> MVAESNSAVAPTANVATSPAHEHFVRVNGGHFELQGKPYVITGVNMWYAAYLGAPNEVGDRDRLAKELDNLKAIGVNNLRVLAVSEKSEINSAVKPAVTNGFGNYDETLLQGLDYLLVELAKRDMTVVLYFNNFWQWSGGMTQYMAWIEGEPVQDPNVTNEWEAFMAKSASFYRSEKAQQEYRKTLEKIITRVNSINGKAYVDDATIMSWQLANEPRPGNSQTTAEEKQIYIDWVHAAAAYIKTLDAHHLVSSGSEGEMGSVNDMQVFIDAHATPDIDYLTYHMWIRNWSWFDKTKPAETWPSAWEKAQNYMRAHIDVAKQLNKPLVLEEFGLDRDMGSYAMDSTTEYRDNYFRGVFELMLASLEQGEPSAGYNIWAWNGYGRTTRANYWWQ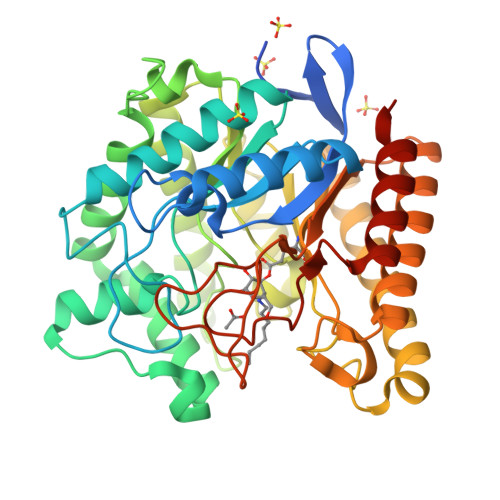EGDDFMGDPPQEEQGMYGVFDTDTSTIAIMKEFNARFQPKLEHHHHHH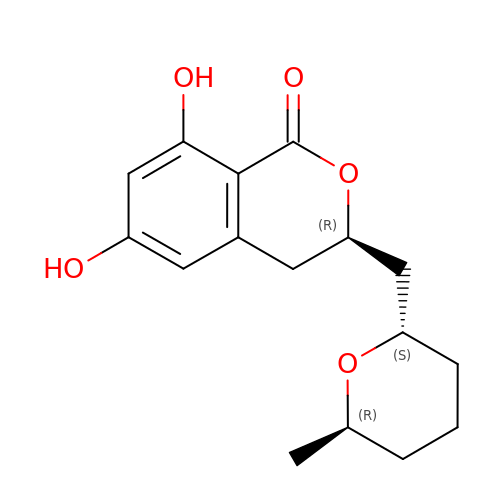(3R)-6,8-dihydroxy-3-{[(2S,6R)-6-methyloxan-2-yl]methyl}-3,4-dihydro-1H-2-benzopyran-1-one | C16 H20 O5 | WOMKDMUZNBFXKG-JIMOISOXSA-N>MSKRLEGKVALVTGGTSGIGLATAKDLAAQGARVIIT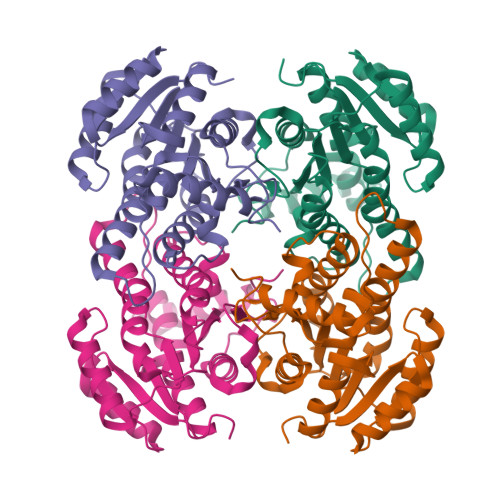GRRQAELDQAVAALGQGVRGVRSDVTRSADLDALFETIRATEGRLDVLFTNAGGGSMAALGEISEQHFDDTFERNVKAVVFTVQKALPLMPQGASIILNGSIAGSTGTQAFSIYGASKAAVRALARSWVLDLKERGIRVNVVSPGSTRTIGLAELGGDTQEGQDGLLAYLASLVPIGRLADPSEIAKVVSFLASDDSSFINGAEITADGGQAQV[4x]> VDPAKEAIMKPQLTMLKGLSDAELKALADFILRIAKQAQEKQQQDVAKAIFQQKGCGSCHQANVDTVGPSLAKIAQAYAGK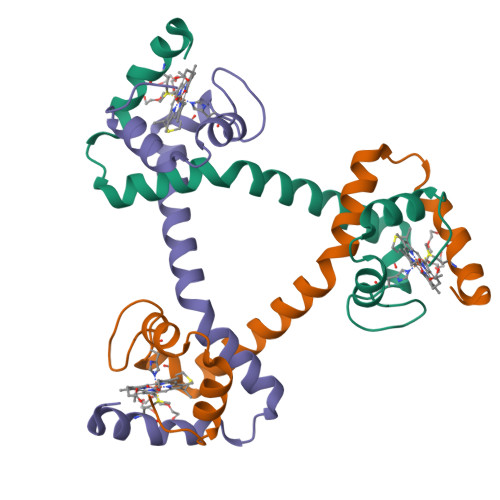EDQLIKFLKGEAPAI1-(4-methylphenyl)sulfonyl-N-(1,3-oxazol-2-ylmethyl)pyrrole-3-carboxamide 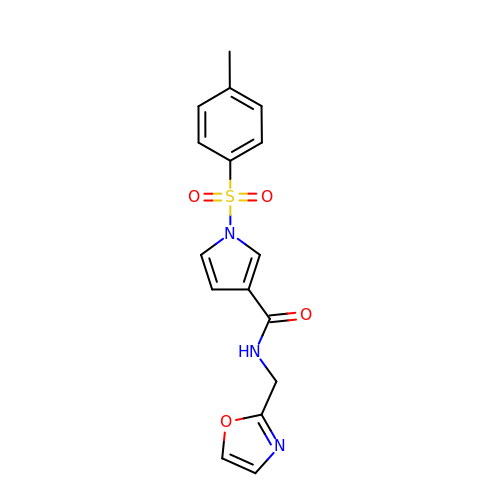| C16 H15 N3 O4 S | ZNWZRQDRLJHYOE-UHFFFAOYSA-N>[2x]MSQKPHLNLIVIGHVDHGKSTLVGRLLMDRGFIDEKTVKEAEEAAKKLGKESEKFAFLLDRLKEERERGV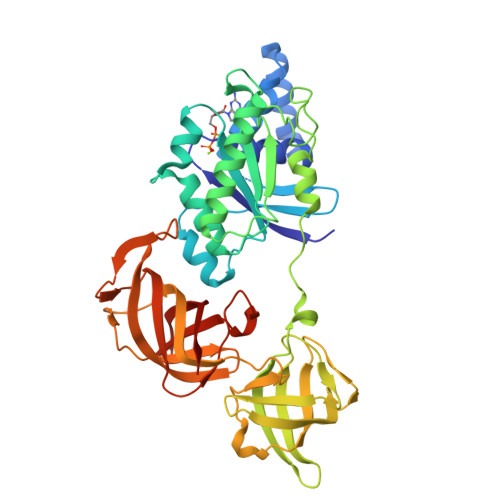TINLTFMRFETKKYFFTIIDAPGHRDFVKNMITGASQADAAILVVSAKKGEYEAGMSVEGQTREHIILAKTMGLDQLIVAVNKMDLTEPPYDEKRYKEIVDQVSKFMRSYGFNTNKVRFVPVVAPSGDNITHKSENMKWYNGPTLEEYLDQLELPPKPVDKPLRIPIQDVYSISGVGTVPVGRVESGVLKVGDKIVFMPAGKVGEVRSIETHHTKMDKAEPGDNIGFNVRGVEKKDIKRGDVVGHPNNPPTVADEFTARIIVVWHPTALANGYTPVLHVHTASVACRVSELVSKLDPRTGQEAEKNPQFLKQGDVAIVKFKPIKPLCVEKYNEFPPLGRFAMRDMGKTVGVGIIVDVKPAKVEIK>[2x]SHMSVSSLLEVVADDLLK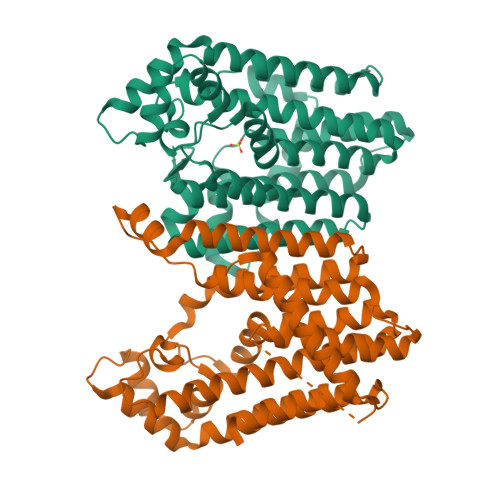LNNNLKSLVGAENPVLVSAAEQIFGAGGKRLRPALVFLVSRATAELAGLLELTTEHQRLAEIIEMIHTASLIHDDVIDDSGMRRGKETIHQLYGTRVAVLAGDFMFAQSSWFLANLENIEVIKLISQVIKDFASGEIKQASTLFDCDITLDDYLLKSYYKTASLIAASTRSAAIFSGVSTAICEQMYEYGRNLGLSFQVVDDILDFTQSAEQLGKPAGSDLAKGNLTAPVIFALQDEPQLREIIDSEFSETNSLATAIELVHRSGGIKRAHELAREKGEIAIQSLQCLPRSEFRSTLENMVKYNLERID> SISQQTVWNQMATVRTPLNFDSSKQSFCQFSVDLLGGGISVDKTGDWITLVQNSPISNLLRVAAWKKGCLMVKVVMSGNAAVKRSDWASLVQVFLTNSNSTEHFDACRWTKSEPHSWELIFPIEVCGPNNGFEMWSSEWANQTS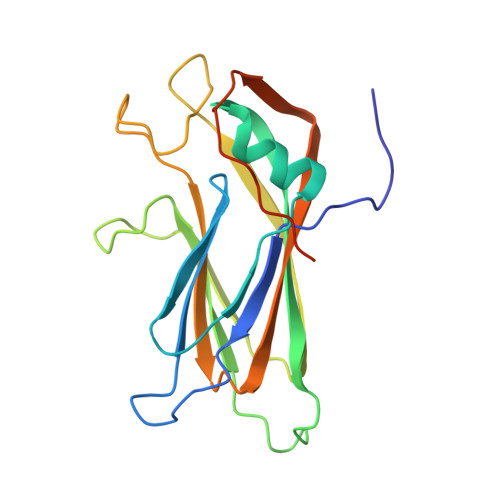WHLSFLVDNPKQSTTFDVLLGISQNFEIAGNTLMPAFSVPQANARSSENAESSA>LVPRGSHMSERADGAQRALAQVRLLWGVCGSFSAVAVPHVNAWLRGTVGVQEIRTVMTAQARALMGPRMIEAVTGHAPVTDWEDHKGGGAAHVALGAWADVLVI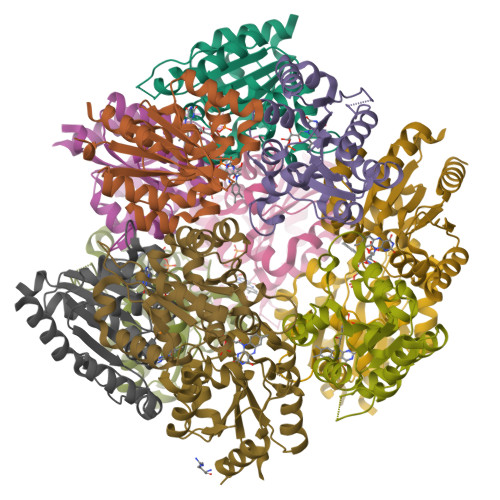LPATANFLAKAAHGIADDVLTATVLAAECPTVIAPVMNAAMWSKPAVQRNVDQLREDGYRIVEPKEGISLTEGRREPGSLGDFQSAISTALIQAAARRTDPRGQ[24x]> MENTENSVDSKSIKNLEPKIIHGSESMDSGISLDNSYKMDYPEMGLCIIINNKNFHKSTGMTSRSGTDVDAANLRETFRNLKYEVRNKNDLTREEIVELMRDVSKEDHSKRSSFVCVLLSHGEAGIIFGTNGPVDLKKITNFFRGDRCRSLTGKPKLFIIQACRGTELDCGIETDSGVDDDMACHKIPVEADFLYAYSTAPGYYSWRNSKDGSWFIQSLCAMLKQYADKLEFMHILTRVNRKVATEFESFSFDATFHAKKQIPCIH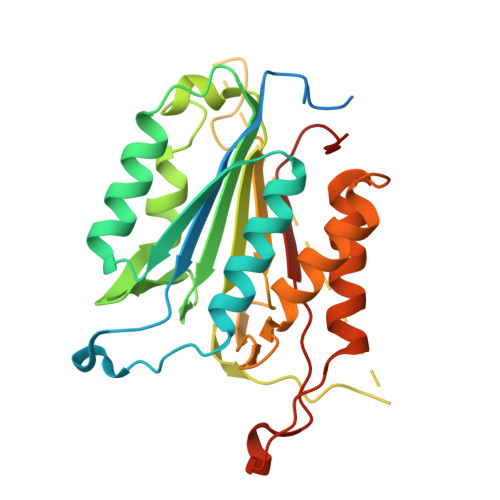SMLTKELYFYH>[4x]MGAALGTGTRLAPWPGRACGALPRWTPTAPAQGCHSKPGPARPVPLKKRGYDVTRNPHLNKGMAFTLEERLQLGIHGLIPPCFLSQDVQLLRIMRYYERQQSDLDKYIILMTLQDRNEKLFYRVLTSDVEKFMPIVYTPTVGLACQHYGLTFRRPRGLFITIHDKGHLATMLNSWPEDNIKAVVVTDGERILGLGDLGCYGMGIPVGKLALYTACGGVNPQQCLPVLLDVGTNNEELLRDPLYIGLKHQRVHGKAYDDLLDEF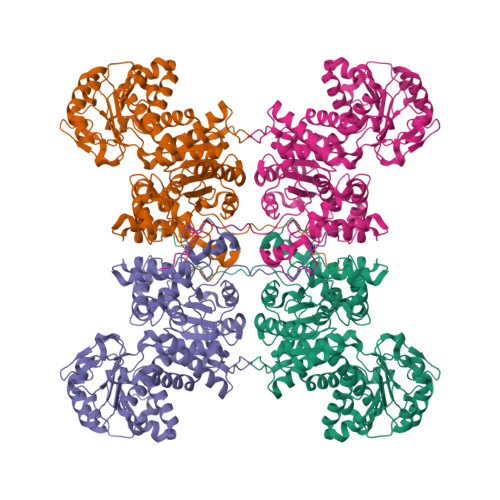MQAVTDKFGINCLIQFEDFANANAFRLLNKYRNKYCMFNDDIQGTASVAVAGILAALRITKNKLSNHVFVFQGAGEAAMGIAHLLVMALEKEGVPKAEATRKIWMVDSKGLIVKGRSHLNHEKEMFAQDHPEVNSLEEVVRLVKPTAIIGVAAIAGAFTEQILRDMASFHERPIIFALSNPTSKAECTAEKCYRVTEGRGIFASGSPFKSVTLEDGKTFIPGQGNNAYVFPGVALGVIAGGIRHIPDEIFLLTAEQIAQEVSEQHLSQGRLYPPLSTIRDVSLRIAIKVLDYAYKHNLASYYPEPKDKEAFVRSLVYTPDYDSFTLDSYTWPKEAMNVQTV>[4x]APAPQPPPILKVFNRPILFDIVSRGSTADLDGLLSFLLTHKKRLTDEEFREPSTGKTCLPKALLNLSNGRNDTIPVLLDIAERTGNMREFINSPFRDIYYRGQTSLHIAIERRCKHYVELLVAQGADVHAQARGRFFQPKDEGGYFYFGELPLSLAACTNQPHIVNYLTENPHKKADMRRQDSRGNTVLHALVAIADNTRENTKFVTKMYDLLLLKCSRLFPDSNLETVLNNDGLSPLMMAAKTGKIGVFQHIIRREVTDEDTRHLSRKFKDWAYGPVYSSLYDLSSLDTCGEEVSVLEILVYNSKIENRHEMLAVEPINELLRDKWRKFGAVSFYINVVSYLCAMVIFTLTAYYQPLEGTPPYPYRTTVDYLRLAGEVITLFTGVLFFFTSIKDLFTKKCPGVNSLFVDGSFQLLYFIYSVLVVVSAALYLAGIEAYLAVMVFALVLGWMNALYFTRGLKLTGTYSIMIQKILFKDLFRFLL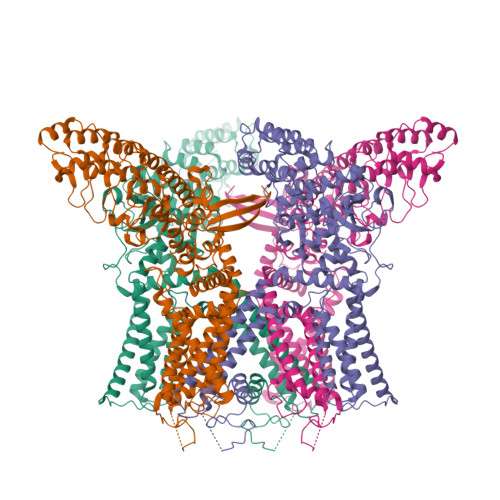VYLLFMIGYASALVTLLNPCTNMKVCDEDQSNCTVPTYPACRDSETFSAFLLDLFKLTIGMGDLEMLSSAKYPVVFILLLVTYIILTFVLLLNMLIALMGETVGQVSKESKHIWKLQWATTILDIERSFPVFLRKAFRSGEMVTVGKSSDGTPDRRWCFRVDEVNWSHWNQNLGIINEDPGK>[2x]ECSVDIQGNDQMQFNTNAHTVDKSCKQFTVNLSHPGNLPKNVMGHNYVLSTAADMQGVVTDGMASGLD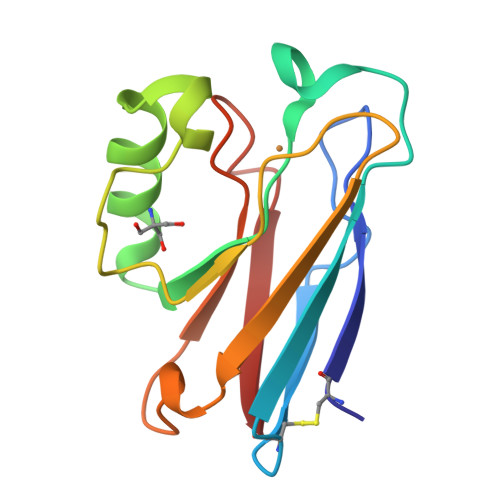KDFLKPDDSRVIAHTKLIGSGEKDSVTFDVSKLKEGEQFMFFCTFPGHSALMKGTLTLK>[2x]SNAEQYHSQV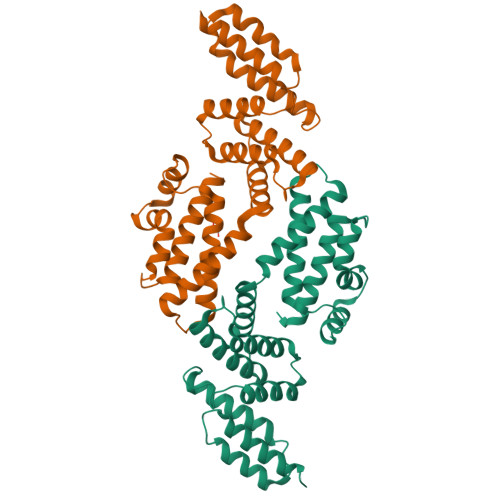VGKIGYIARCMQTIDPENNLKKIREDYQDVLIWAEKNYRFEEILEASKSGKCPNDLDALSRRSLILQELLRLVSSISPFKMKLDLIESQYEKMKQHVNLWKSDYHVKLNQLNQLTDYLKNAAPTPKNNFLRAMTSVLQMQIAQYGITEDNEGINQLFKLGLHLLAMANEKIDEQYHLFKGYVKDQPEESPFEGILPAEDQKILVKTMIDYAMPKLSSKVLQDKLSALSSSDVLTKTLLDSIDRIVKENEKLNALSK> MGSSHHHHHHSQDPMMEYKIVENGLTYRIGNGASVPISNTGELIKGLRNYGPYEVPSLKYNQIALIHNNQFSSLINQLKSQISSKIDEVWHIHNINISEFIYDSPHFDSIKSQVDNAIDTGVDGIMLVLPEYNTPLYYKLKSYLINSIPSQFMRYDILSNRNLTFYVDNLLVQFVSKLGGKPWILNVDPEKGSDIIIGTGATRIDNVNLFCFAMVFKKDGTMLWNEISPIVTSSEYLTYLKSTIKKVVYGFKKSNPDWDVEKLTLHVSGKRPKMKDGETKILKETVEELKKQEMVSRDVKYAILHLNETHPFWVMGDPNNRFHPYEGTKVKLSSKRYLLTLLQPYLKRNGLEMVTPIKPLSVEIVSDNWTSEEYYHNVHEILDEIYYLSKMNWRGFRSRNLPVTVNYPKLVAGIIANVNRYGGYPINPEGNRSLQTNPWFL;> MGSSHHHHHHSQDPMEIPLSSGNVNTPDVRSSGILYINIYPIVNYPETIKVSAIPYYEEFLPGKWKKRIGDLIYLYGYGIENEFDEIDNSNALFGKIFRKYLLDILSENIATPWQLKELGSTLRLVKEITENYEFSNIIKLQYELIINVHHWQNTNFGIIVDLKINILDRENNQRISYTKIKDKYGESVKKKIWVSVQAFHRHLTPEGKKYATAMRDKFNLLTGLLKEAFGSSEDEKTFSTPDGEIKIVFKPLEIVEVSNNDGI

Here we focus on the prokaryotic Argonaute AfAgo from Archaeoglobus fulgidus DSM4304. Although phylogenetically classified as a long-B pAgo, AfAgo contains only MID and catalytically inactive PIWI domains, akin to short pAgos. We show that AfAgo forms a heterodimeric complex with a protein encoded upstream in the same operon, which is a structural equivalent of the N-L1-L2 domains of long pAgos. This complex, structurally equivalent to a long PAZ-less pAgo, outperforms standalone AfAgo in guide RNA-mediated target DNA binding.

Next, we obtained cryo-EM structures of the fAfAgo complex with two variants of gRNA/tDNA heteroduplexes: g30/t51 (30 nt gRNA, 51 nt tDNA, final resolution 2.83 Å) and g17/t17 (17 nt gRNA, 17 nt gDNA, resolution 3.56 Å), and a 2.5 Å crystal structure of fAfAgo bound to a 15 nt 5′-phosphorylated ssDNA oligonucleotide. The crystal structure contains fragments of two partially annealed non-self-complementary DNA oligonucleotide strands forming a short (3 bp) guide/target-like dsDNA region. Relative orientation of AfAgo and AfAgo-N proteins in the crystal structure slightly differs from that in cryo-EM structures obtained with longer gRNA/tDNA heteroduplexes (RMSD values 1.9–2.3 Å). A similar set of contacts to bases and backbone is also observed in the crystal structure of fAfAgo bound to a short DNA duplex fragment. The AfAgo subunit, both standalone and AfAgo-N-bound, anchors the 5′–phosphorylated terminus of the guide strand in a conserved MID domain pocket, disrupts the g1:t1 (the first guide strand and the complementary target strand nucleotides) base pair by placing the g1 adenine and the t1 thymine bases into separated protein pockets, and makes similar contacts to the neighboring g2:t2 and g3:t3 base pairs. The AfAgo-N subunit sterically masks the AfAgo surface that was previously implicated in AfAgo homodimerization, making AfAgo oligomerization across this surface unlikely. Taken together, structures presented here demonstrate that fAfAgo heterodimer preserves the g1:t1 base pair recognition mechanism previously demonstrated for the standalone AfAgo, but unlike the isolated AfAgo subunit, fAfAgo binds the guide/target heteroduplex in a specialized cleft in a similar manner as the structurally related long-B pAgos.> SEGITDIEESQIQTNYQKVVYKFDDMELDEQLLRGVFGYGFEEPSAIQQRAIMPIIEGHDVLAQAQSGTGKTG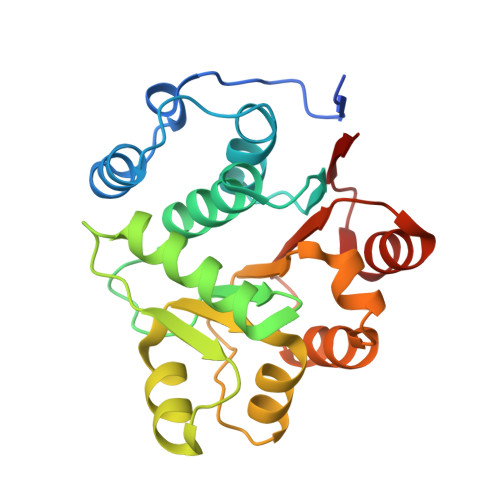TFSIAALQRIDTSVKAPQALMLAPTRELALQIQKVVMALAFHMDIKVHACIGGTSFVEDAEGLRDAQIVVGTPGRVFDNIQRRRFRTDKIKMFILDEADEMLSSGFKEQIYQIFTLLPPTTQVVLLSATMPNDVLEVTTKFMRNPVRILV RRR-ALPHA-TOCOPHERYLQUINONE | C29 H50 O3 | 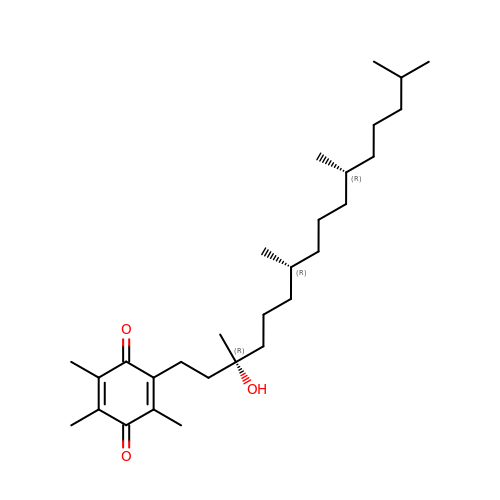LTVDFSLWFKLJDQ-IEOSBIPESA-N> GGHHHHHHGIFKPEELRQALMPTLEALYRQDPESLPFRQPVDPQLLGIPDYFDIVKSPMDLSTIKRKLDTGQYQEPWQYVDDIWLMFNNAWLYNRKTSRVYKYCSKLSEVFEQEIDPVMQSLGYCCGRKLEFSPQTLCCYGKQLCTI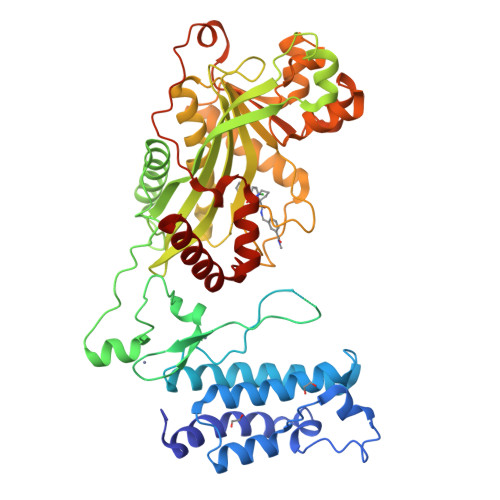PRDATYYSYQNRYHFCEKCFNEIQGESVSLGDDPSQPQTTINKEQFSKRKNDTLDPELFVECTECGRKMHQICVLHHEIIWPAGFVCDGCLKKSARTRKENKFSAKRLPSTRLGTFLENRVNDFLRRQNHPESGEVTVRVVHASDKTVEVKPGMKARFVDSGEMAESFPYRTKALFAFEEIDGVDLCFFGMHVQEYGSDCPPPNQRRVYISYLDSVHFFRPKCLRTAVYHEILIGYLEYVKKLGYTTGHIWACPPSEGDDYIFHCHPPDQKIPKPKRLQEWFKKMLDKAVSERIVHDYKDIFKQATEDRLTSAKELPYFEGDFWPNVLEESIKESGGSGQKLYATMEKHKEVFFVIRLIAGPAANSLPPIVDPDPLIPCDLMDGRDAFLTLARDKHLEFSSLRRAQWSTMCMLVELHTQSQD>MRAVRLVEIGKPLSLQEIGVPKPKGPQVLIKVEAAGVCHSDVHMRQGRFGNLRIVEDLGVKLPVTLGHEIAGKIEEVGDEVVGYSKGDLVAVNPWQGEGNCYYCRIGEEHLCDSPRWLGINFDGAYAEYVIVPHYKYMYKLRRLNAVEAAPLTCSGITTYRAVRKASLDPTKTLLVVGAGGGLGTMAVQIAKAVSGATIIGVDVREEAVEAAKRAGADYVINASMQDPLAEIRRITESKGVDAVIDLNYSEKTLSVYPKALAKQGKYVMVGLFGADLHYHAPLITLSEIQFV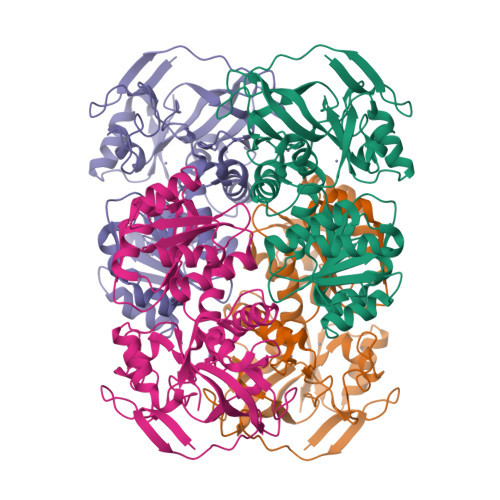GSLVGNQSDFLGIMRLAEAGKVKPMITKTMKLEEANEAIDNLENFKAIGRQVLIP[6x]3-[3-(dimethylamino)phenyl]benzoic 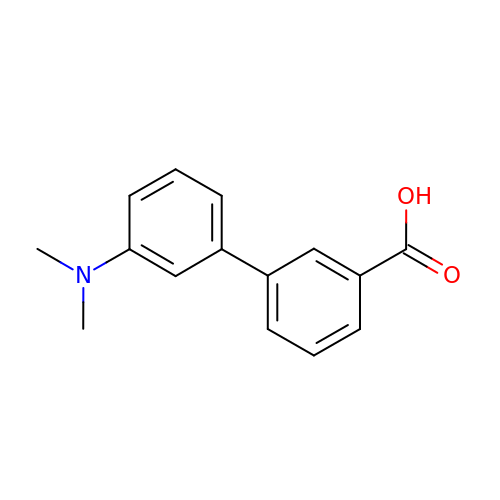acid | C15 H15 N O2 | IGKUVSHRCBIVKZ-UHFFFAOYSA-N>VQREVLDLGELISEFEVLLRRLLREDVKLITDYGRDLPQVRAD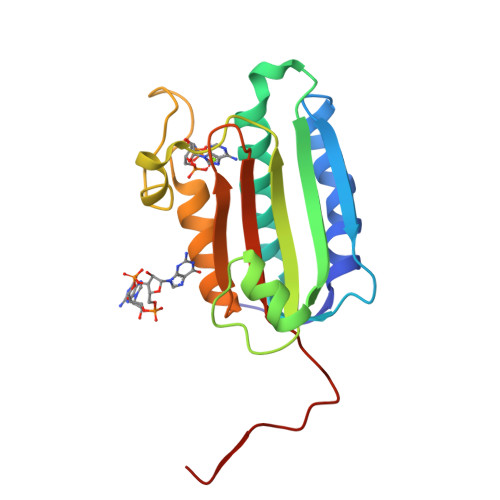KSQLETAVMNLAVNARDAVRAAKGGGVVRIRTARLTRDEAIQLGFPAADGDTAFIEVSDDGPGIPPDVMGKIFDPFFTTKPVGEGTGLGLATVYGIVKQSDGWIHVHSRPNEGAAFRIFLPVYEAPAALEHHHHHH[2x]> GSPGISGGGGGILDSMVEKEEPKEEEKLGKLQYSLDYDFQNNQLLVGIIQAAELPALDMGGTSDPYVKVFLLPDKKKKFETKVHR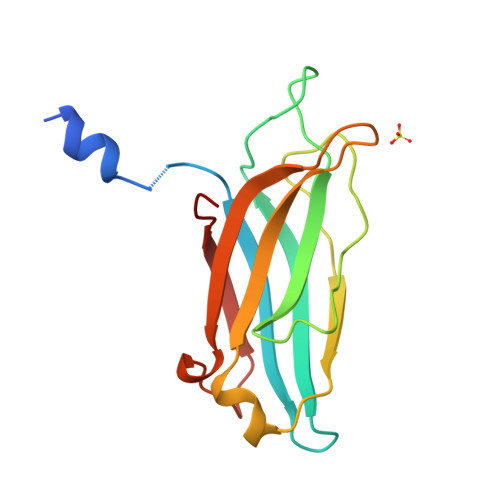KTLNPVFNEQFTFKVPYSELGGKTLVMAVYDFDRFSKHDIIGEFKVPMNTVDFGHVTEEWRDLQSAE1-cyclopentyl-N-[(2S,3R)-3-hydroxy-1-phenyl-4-{[3-(trifluoromethyl)benzyl]amino}butan-2-yl]-6-oxo-5-(2-oxopyrrolidin-1-yl)-1,6-dihydropyridine-3-carboxamide 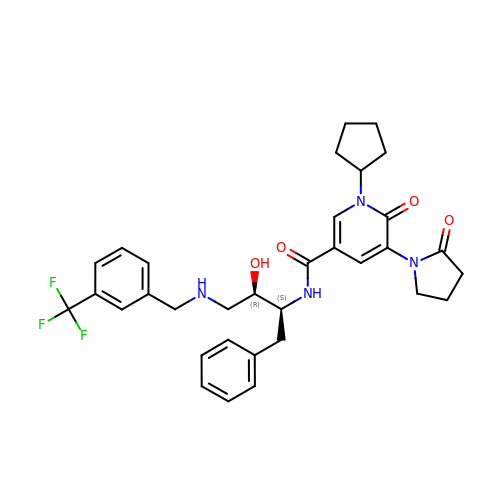| C33 H37 F3 N4 O4 | QKLJNYJRYSKKKP-LMSSTIIKSA-N> LRNTKHEISEMNRMIQRLRAEIDNVKKQCANLQNAIADAEQRGELALKDARNKLAELEEALQKAKQDMARLLREYQELMNTKLALDVEIATYRKLLE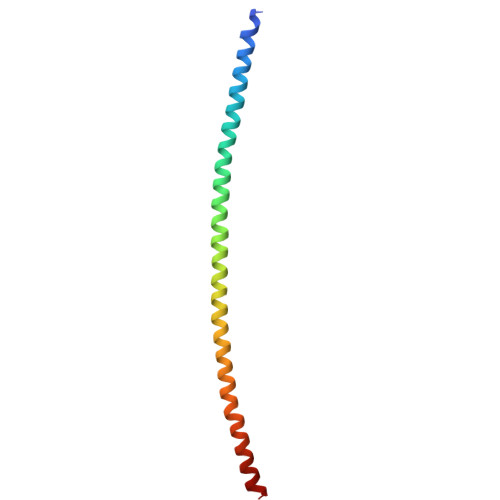G> EKSKVAGSAAAASAAAASDGSSCDHGPGAISRRSHITLPAYFAGTTENWVSCAGCGVTLGHSLGAFLSLAVAGHSGSDFALASTSFARSAKGKRTDYVEVFDPVTFLPIADIELPDAPRFSVGPRVHIIGNCASSACLLFFLFGSSAAAGLSVPGASDDQLTKSASCFHIHPGAAATHYLGSCPASLAASDLAAAPAAAGIVGAQCTGAQNCSSQAAQANYPGMLVWA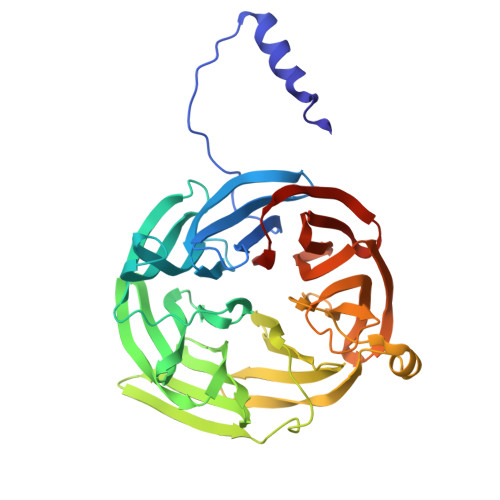VASSILQGDIPAAGATMKAAIDGNESGRKADNFRSAGFQMVAKLKNTDGIMILTVEHSRSCLAAAENTSSVTASVGQTSGPISNGHDSDAIIAAQDGASDNYANSAGTEVLDIYDAASDQDQSSVELDKGPESLSVQNEA The mammalian global genome nucleotide excision repair (NER) factor, xeroderma pigmentosum C (XPC)–RAD23B complex (hereafter XPC), in particular, faces a difficult challenge. Once bound to a lesion, XPC recruits the multi-subunit transcription factor IIH (TFIIH) that verifies the lesion, which ultimately coordinates the assembly of NER factors, causing excision of a lesion-containing single-stranded DNA and repair synthesis that restores the duplex. The previous crystal structures of the yeast XPC orthologue, Rad4, bound to model lesions have shown that Rad4 and, by analogy, XPC recognize the damaged DNA site by inserting a β-hairpin into DNA duplex and flipping out damage-containing nucleotide pairs to form an ‘open’ conformation. In this conformation, Rad4 interacts exclusively with the two nucleotides on the undamaged strand without making specific contacts with the two damaged residues of the model UV lesion.

The 2AP fluorescence of the mismatch DNA in complex with either of the Rad4 mutants shows a temperature dependence very similar to that of free DNA. These results contrast with the behaviour of the wild-type Rad4–mismatch DNA complex, which showed an increase in fluorescence emission intensity with increasing temperature (left). Furthermore, no relaxation kinetics (other than the T-jump recovery kinetics) was observed with these β-hairpin mutants. The results indicate that the β-hairpin is indeed critical for forming and stabilizing the ‘open’ conformation, consistent with other studies (refs 8, 18).

> GSSRAMGNEVAGVEDISVEITPSSKRNSDARRTSRNCSSNEERKRRKYFHMLYLVCLMVHGFIRNEWINSKRLSRKLSNLVPEKVFELLHPQKDEELPLRSTRKLLDGLKKCMELWQKHWKITKKYDNEGLYMRTWKEIEMSANNKRKFKTLKRSDFLRAVSKGHGDPDISVQGFVAMLRACNVNARLIMSCQPPDFTNMKIDTSLNGNNAYKDMVKYPIFWCEVWDKFSKKWITVDPVNLKTIEQVRLHSKLAPKGVACCERNMLRYVIAYDRKYGCRDVTRRYAQWMNSKVRKRRITKDDFGEKWFRKVITALHHRKRTKIDDYEDQYFFRRDESEGIPDSVQDLKNHPYYVLEQDIKQTQIVKPGCKECGYLKVHGKVGKVLKVYAKRDIADLKSARQWYMNGRILKTGSRCKKVIKRTVGRPKGEAEEEDERLYSFEDTELYIPPLASASGEITKNTFGNIEVFAPTMIPGNCCLVENPVAIKAARFLGVEFAPAVTSFKFPVLSGIVVAKWLREAIETAIDGIEFI;> GSGNASSGALGTTGGATDAAQGGPPGSIGLTVEDLLSLRQVVSGNPEALAPLLENISARYPQLREHIMANPEVFVSMLLEAVGDNMQDVMEGADDMVEGEDIEVTGEAAAAGLGQGEGEGSFQVDYTPEDDQAISRLCELGFERDLVIQVYFACDKNEEAAANILFSDHAD> MTQAKAKHADVPVNLYRPNAPFIGKVISNEPLVKEGGIGIVQHIKFDLTGGNLKYIEGQSIGIIPPGVDKNGKPEKLRLYSIASTRHGDDVDDKTISLCVR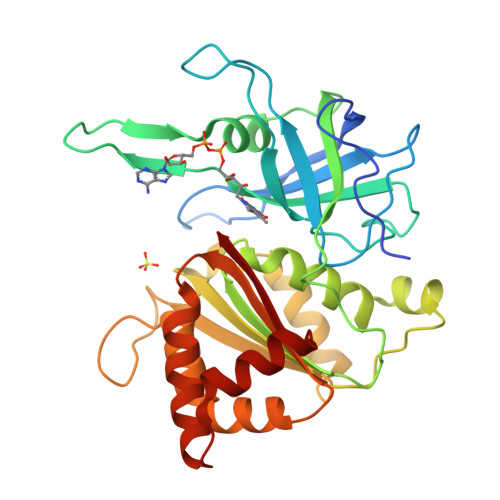QLEYKHPESGETVYGVCSTYLTHIEPGSEVKITGPVGKEMLLPDDPEANVIMLATGTGIAPMRTYLWRMFKDAERAANPEYQFKGFSWLVFGVPTTPNILYKEELEEIQQKYPDNFRLTYAISREQKNPQGGRMYIQDRVAEHADQLWQLIKNQKTHTYICGLRGMEEGIDAALSAAAAKEGVTWSDYQKDLKKAGRWHVETW>GAMGWCIFIYNLGQDADEGILWQMFGPFGAVTNVKVIRDFNTNKCKGFGFVTMTNYEEAAMAIASLNGYRLG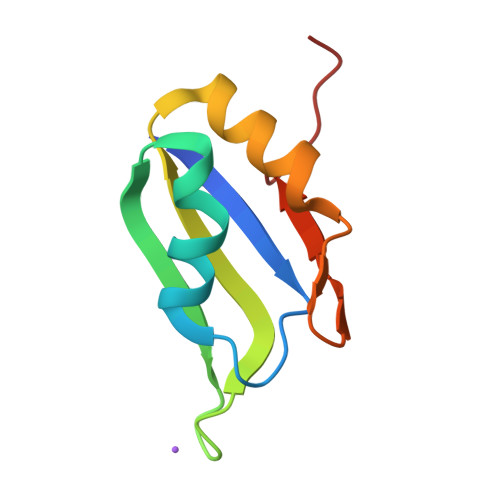DKILQVSFKTNKSHK[3x]> GSEIAVQNPLVSERLELSVLYKEYAEDDNIYQQKIKDLHKKYSYIRKTRPDGNCFYRAFGFSHLEALLDDSKELQRFKAVSAKSKEDLVSQGFTEFTIEDFHNT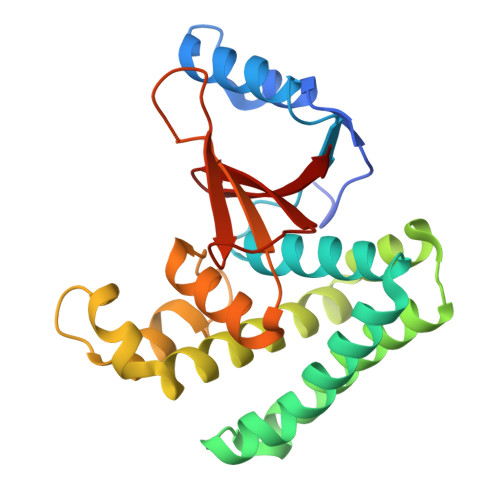FMDLIEQVEKQTSVADLLASFNDQSTSDYLVVYLRLLTSGYLQRESKFFEHFIEGGRTVKEFCQQEVEPMCKESDHIHIIALAQALSVSIQVEYMDRGEGGTTNPHIFPEGSEPKVYLLYRPGHYDILYK>[4x]RSELRFDPGTSNRNFRIAASDFGQALMLPRLYATLEETAPQVRVTGVNLRHGPLVEELESGSIDIAFGGFPTLSAGIKTQTLFREEYVCVMRQSHPALTHGLDLEAFRQCRHIIVTAHEFNHVHEQVEARLLELLPPESIRFTTENFLVSAVIAEETDVILTIPSRLARWFANRGGLTIFPVPIELPSIEVKQYWHERYDKDPGNIWLRRVIAKIGFQNPPAE

PcpR and TcpR belong to the LysR transcriptional regulator (LTTR) and are responsible for controlling the degradation of PCP and 2,4,6-TCP, respectively, although their precise mechanism of transcriptional control is not well defined. In general, the LysR family transcription factors consist of an N-terminal DNA-binding domain (DBD) and a C-terminal inducer-binding domain (IBD). The monomeric structure of the PcpR inducer-binding domain contains two nucleotide-binding (or Rossmann fold) motifs connected by a hinge region. The PcpR dimer was established by interactions between β-strands and α-helices from each monomer.

The complex structure of PcpR with PCP displayed the clear electron density for two bound PCP molecules located in two inducer binding cavities (IBC). The first cavity (IBC1) was located underneath a hinge region between two lobes of the inducer-binding domain and the nearby second cavity (IBC2) was rather exposed to the surface. In IBC1, the PCP molecule was confined in a relatively hydrophobic pocket formed by residues S104, F106, L110, F151, F167, Y171, H206, H208, F231, P248, and V275. In contrast, the imidazole ring of H206 was pushed away in the PCP complex structure and not involved in a hydrogen bond network probably due to steric adjustment for the bulkier PCP. The second binding cavity (IBC2), which was unique to the PCP complex, was located near the dimer interface between α1 of RDI and α9 of RDII. The pocket is formed from residues F106, L110, R114, W254 and P305. PCP interacts with the indole sidechain of W254 through π-stacking, and the oxyanion of PCP interacts electrostatically with the guanidinium sidechain of R114. Additionally, two residues from the adjacent monomer at the dimer interface, V236 and E240, contributed to the second PCP-binding cavity. The titration curve of PCP displayed a two-binding site mode, one tight and the other much weaker. The second binding site for PCP had a Kd2 = 70 µM, ΔH2 = −9.0 kcal/mol, and ΔS2 = −11.0 cal·mol−1·K−1. This second binding event observed in ITC measurements correlates well with observed PCP at IBC2 in our complex crystal structures.(2S)-2-(acetylamino)-N-methyl-4-[(R)-methylsulfinyl]butanamide | C8 H16 N2 O3 S | 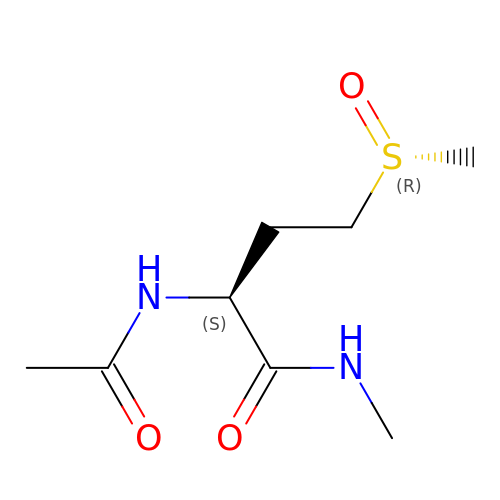HOKSMYPIXLKSMM-JKYUHCHBSA-N As a proof of concept, we used this platform to identify both known and novel L- and D-amino acid peptide binders to the well-characterized model target, streptavidin. All peptides bind within or near the biotin binding pocket of streptavidin formed by two surface loops [1/2 (amino acids 22–28) and 3/4 (amino acids 42–52)], and by antiparallel β-sheets involved in an extensive polar interaction network, in which residues Ser88 and Thr90 of β-strand 6 play a major role. The surface loops of streptavidin are flexible: upon biotin binding they undergo a conformational change to form a closed conformation, but to accommodate the peptide ligands, loop 3/4 is dislocated by 13–16 Å from the biotin closed form to adopt a well-defined peptide-specific structure. All eight L- and D-peptides discovered in this work bind to the same pocket of streptavidin in distinctive binding modes suggesting (1) the rich malleability of L- and D-peptides and (2) the ability of streptavidin itself to adjust the flexible loop to accommodate multiple peptides with diverse sequences and conformations.

From these “secondary” peptide families identified in the initial screen, we chose three 5-mer “hot spot” sequences: LAEYH, PAWAH, and FDEWL. We used a series of array peptide libraries rationally designed around each of these sequences to successfully evolve the three sequences to 12-mer L-peptides. The AFPDYLAEYHGG L-peptide had the lowest Kd value, 43 nM, among all peptides discovered in this work. One L-peptide, AFPDYLAEYHGG, showed a Kd of 43 nM—a 100-fold improvement over the HPQ peptide also developed in this study, and 1,000-fold greater than Strep-tag II HPQ. Strong correlation between specificity in the substitution plots and co-crystal data was also observed for the AFPDYLAEYHGG peptide (the highest affinity for streptavidin in SPR measurements) and the RDPAPAWAHGGG peptide (the longest stretch of highly specific amino acids between positions 2 and 11) (respectively). Although these effects cannot be completely excluded, comparing the substitution plots with the co-crystal structures for each peptide revealed an excellent correlation between the binding specificity of the preferred amino acids and their relative contribution to the interactions with streptavidin in the co-crystal structure.

>[4x]MRKIVVAAIAVSLTTVSITASASADPSKDSKAQVSAAEAGITGTWYNQLGSTFIVTAGADGALTGTYESAVGNAESRYVLTGRYDSAPATDGSGTALGWTVAWKNNYRNAHSATTWSGQYVGGAEARINTQWLLTSGTTEANAWKSTLVGHDTFTKVKPSAASIDAAKKAGVNNGNPLDAVQQ;>[4x]AFPDYLAEYHGGX> RICFNHQSSQPQTTKTCSPGESSCYNK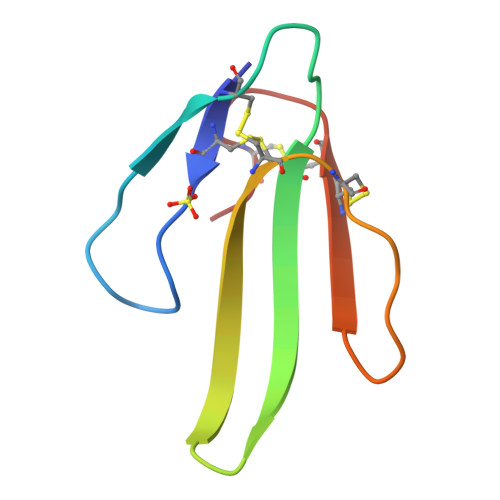QWSDFRGTIIERGCGCPTVKPGIKLSCCESEVCNN>[2x]EAEAYVEFTTVNVNYPEGEVVGVSVLGIESFRGVPFAQPPVGNLRLKPPVRYTENIGTK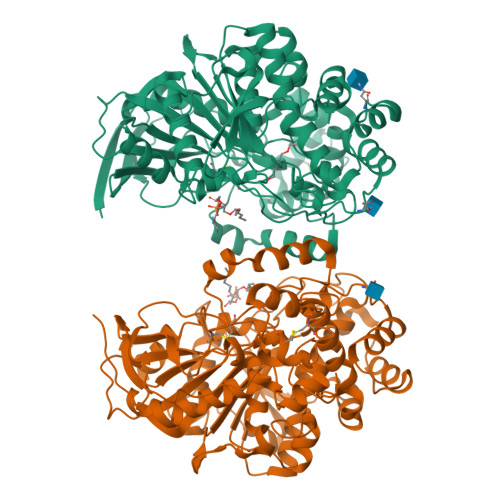DTTGIGPSCPQMYLSTGNGELLFQLVGNLINIPLFQTATLSSEDCLTLNIQRPAGTTSNSSLPVLFWIFGGGFELGTNQYYDGIDLLTEGISLGEPFIFVAINYRVGGFGFLGGKEIKADGSSNLGLLDQRIALEWVADNIASFGGDPSKVTIWGESAGSISVFDQMALYGGNNKYKGKALFRGGIMNSGSVVPAAPVDGVKAQAIYDHVVSEAGCAGTSDTLACLRTVDYTKFLTAVNSVPGIVSYSSIALSYLPRPDGVVLIDSPEEIVKNKQYAAVPMIIGDQEDEGTLFAVLPNNITSTAKIVQYFQDLYFYNATKEQLTAFVNTYPTDITAGSPFNTGIFNELYPGFKRLAAILGDMTFTLARRAFLQLCSEVNPDVPSWSYLASYDYGFPFLGTFHATDILQVFYGVLPNYASGSIQKYYINFVTTGDPNKGAAVDIQWPQWSAKKNILQIYATKAVIVADNFRAKSYEYLYNNWGIFRI Fast synaptic transmission throughout the central and peripheral nervous system is mediated by pentameric ligand-gated ion channels (pLGICs), also referred to as Cys-loop receptors. The binding of a neurotransmitter initiates a cascade of protein motions that lead to transitions between resting, open, and desensitized conformations. Here, we show in electrophysiological recordings that desensitization in GLIC, a prokaryotic pH-gated pLGIC, is enhanced in the presence of DHA. GLIC has previously been crystallized in its resting (closed) and putative open states, however, the desensitized state of the channel has been structurally elusive.

To better understand the mechanism of DHA action and to attempt trapping GLIC in a desensitized conformation, co-crystals of GLIC were grown in the presence of 50 μM of DHA under acidic conditions, similar to those previously reported for GLIC wt. (A) A side-view of the GLIC-pH4-DHA structure at pH 4.0 solved to 3.25 Å resolution with a bound DHA molecule shown in stick representation. Well-defined electron density was found for DHA in all the subunits in a pocket at the channel periphery; lined by M4, the M2-M3 linker, and the β6-β7 loop. The DHA molecule appears bent with a twisted/curled orientation, and makes a salt-bridge interaction with an arginine sidechain (Arg118) in the β6-β7 loop. However, it must be noted that the density for the DHA tail is not resolved beyond C13, and therefore was not built in the model. The R118A mutant showed robust pH-induced currents in oocytes, however in comparison to GLIC wt, the current decay was much less affected by 50 μM DHA. In this new M2 conformation, the pore is funnel-shaped with the hydrophobic extracellular-end (Ala13′ to Thr20′) wide-open to a pore radius greater than 5 Å, reminiscent of the GLIC-pH4 structure, while the polar intracellular-half (between Ile9′ and Thr2′) is constricted to 2.5 Å, resembling the GLIC-pH7 closed structure. In contrast, in the GLIC-pH4-DHA structure, while the extracellular end remains open, the intracellular-half of M2 (lined by Ile9′, Ser 6′, and Thr2′) undergoes constriction, with the largest effect seen at Ile9′ (pore radii ~2.5 Å). In contrast, the GLIC-pH4-DHA structure shows a distinctly different hydration profile at the intracellular half of the pore, with loss of densities for water and ions. We therefore suggest that the GLIC-pH4-DHA structure represents a desensitized conformation (perhaps a lipid-induced, deeper state), where ion permeation is occluded in the intracellular-end of M2 below the 9′ position.

>VSPPPPIADEPLTVNTGIYLIECYSLDDKAETFKVNAFLSLSWKDRRLAFDPVRSGVRVKTYEPEAIWIPEIRFVNVENARDADVVDISVSPDGTVQYLERFSARVLSPLDFRRYPFDSQTLHIYLIVRSVDTRNIVLAVDLEKVGKNDDVFLTGWDIESFTAVVKPANFALEDRLESKLDYQLRISRQYFSYIPNIILPMLFILFISWTAFWSTSYEANVTLVVSTLIAHIAFNILVETNLPKTPYMTYTGAIIFMIYLFYFVAVIEVTVQHYLKVESQPARAASITRASRIAFPVVFLLANIILAFLFF[5x]>MEESRADGRNPNQLRPFSCTRNPLDRAHGSARWAQGDTIVLAAVYGPKPGTRKGENPEKASIEVVWKPMTGQIGKQEKEYEMTLKRTLQSICLLTVHPNTTTSVILQVVGNDGSLLPCAINACCAALVFAGIPLKHLAVAIGCGVLEDGEVI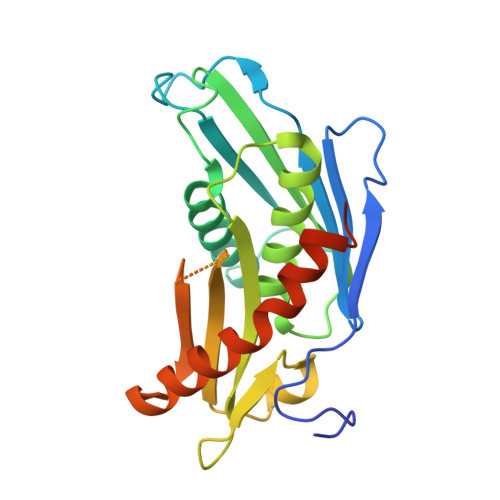LDTNKAEEQQLKSFAHLVFPNSRKSASSKEPNQKEEDSERGLITSITHGVMSEEDYFSCIERGLAASSRISDFMRTTLQKQAPGDVLEHHHHHH[3x]>[2x]MPHFTVTKVEDPEEGAAASISQEPSLADIKARIQDSDEPDLSQNDITGEHSQLLDDGHKKARNAYLNNSNYEEGDEYFDKNLALFEEEMDTRPKVSSLLNRMANYTNLTQGAKEHEEAENITEGKKKPTKTPQMGTFMGVYLPCLQNIFGVILFLRLTWVVGTAGVLQAFAIVLICCCCTMLTAISMSAIATNGVVPAGGSYFMISRALGPEFGGAVGLCFYLGTTFAAAMYILGAIEIFLVYIVPRAAIFHSDDALKESAAMLNNMRVYGTAFLVLMVLVVFIGVRYVNKFASLFLACVIVSILAIYAGAIKSSFAPPHFPVCMLGNRTLSSRHIDVCSKTKEINNMTVPSKLWGFFCNSSQFFNATCDEYFVHNNVTSIQGIPGLASGIITENLWSNYLPKGEIIEKPSAKSSDVLGSLNHEYVLVDITTSFTLLVGIFFPSVTGIMAGSNRSGDLKDAQKSIPIGTILAILTTSFVYLSNVVLFGACIEGVVLRDKFGDAVKGNLVVGTLSWPSPWVIVIGSFFSTCGAGLQSLTGAPRLLQAIAKDNIIPFLRVFGHSKANGEPTWALLLTAAIAELGILIASLDLVAPILSMFFLMCYLFVNLACALQTLLRTPNWRPRFRYYHWALSFMGMSICLALMFISSWYYAIVAMVIAGMIYKYIEYQGAEKEWGDGIRGLSLSAARFALLRLEEGPPHTKNWRPQLLVLLKLDEDLHVKHPRLLTFASQLKAGKGLTIVGSVIVGNFLENYGEALAAEQTIK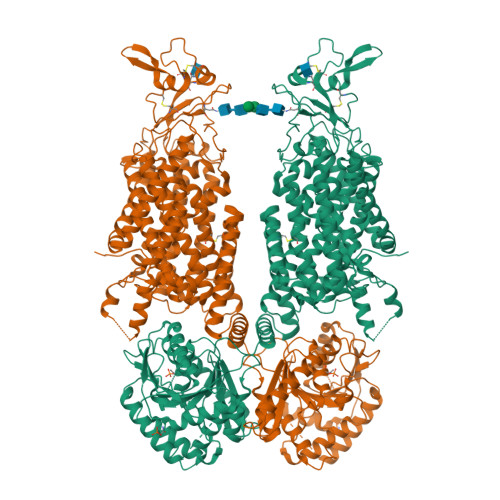HLMEAEKVKGFCQLVVAAKLREGISHLIQSCGLGGMKHNTVVMGWPNGWRQSEDARAWKTFIGTVRVTTAAHLALLVAKNISFFPSNVEQFSEGNIDVWWIVHDGGMLMLLPFLLKQHKVWRKCSIRIFTVAQLEDNSIQMKKDLATFLYHLRIEAEVEVVEMHDSDISAYTYERDLMMEQRSQMLRHMRLSKTERDREAQLVKDRNSMLRLTSIGSDEDEETETYQEKVHMDWTKDKYMASRGQKAKSMEGFQDLLNMRPDQSNVRRMHTAVKLNEVIVNKSHEAKLVLLNMPGPPRNPEGDENYMEFLEVLTEGLERVLLVRGGGSEVITIYS N-(trifluoroacetyl)-L-leucyl-N-[4-(trifluoromethyl)phenyl]-L-alaninamide | C18 H21 F6 N3 O3 | 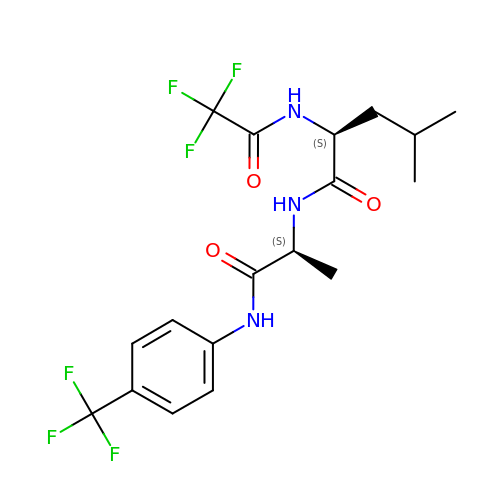COFHEZKAONGFAP-GWCFXTLKSA-N>[2x]VEGRFQLVAPYEPQGDQPQAIAKLVDGLRRGVKHQTLLGATGTGKTFTISNVIAQVNKPTLVIAHNKTLAGQLYSELKEFFPHNAVEYFVSYYDYYQPEAYVPQTDTYIEKDAKINDEIDKL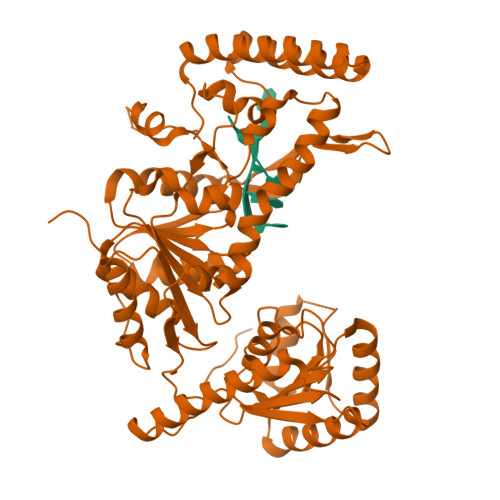RHSATSALFERRDVIIVASVSCIYGLGSPEEYRELVVSLRVGMEIERNALLRRLVDIQYDRNDIDFRRGTFRVRGDVVEIFPASRDEHCIRVEFFGDEIERIREVDALTGEVLGEREHVAIFPASHFVTREEKMRLAIQNIEQELEERLAELRAQGKLLEAQRLEQRTRYDLEMMREMGFCSGIENYSRHLALRPPGSTPYTLLDYFPDDFLIIVDESHVTLPQLRGMYNGDRARKQVLVDHGFRLPSALDNRPLTFEEFEQKINQIIYVSATPGPYELEHSPGVVEQIIRPTGLLDPTIDVRPTKGQIDDLIGEIRERVERNERTLVTTLTKKMAEDLTDYLKEAGIKVAYLHSEIKTLERIEIIRDLRLGKYDVLVGINLLREGLDIPEVSLVAILDADKEGFLRSERSLIQTIGRAARNANGHVIMYADTITKSMEIAIQETKRRRAIQEEYNRKHGIVPRTVKKEIRDVIRATYAAEETEMYEAKPAAAMTKQEREELIRTLEAEMKEAAKALDFERAAQLRDIIFELKAEG>[2x]ATTYNAVVSKSSSDGKTFKTIADAIASAPAGST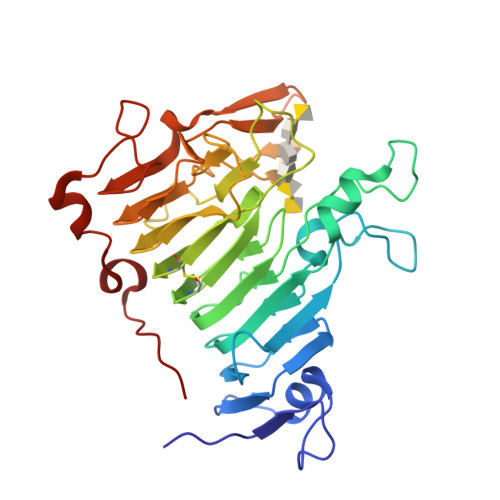PFVILIKNGVYNERLTITRNNLHLKGESRNGAVIAAATAAGTLKSDGSKWGTAGSSTITISAKDFSAQSLTIRNDFDFPANQAKSDSDSSKIKDTQAVALYVTKSGDRAYFKDVSLVGYQATLYVSGGRSFFSDCRISGTVDFIFGDGTALFNNCDLVSRYRADVKSGNVSGYLTAPSTNINQKYGLVITNSRVIRESDSVPAKSYGLGRPWHPTTTFSDGRYADPNAIGQTVFLNTSMDNHIYGWDKMSGKDKNGNTIWFNPEDSRFFEYKSYGAGATVSKDRRQLTDAQAAEYTQSKVLGDWTPTLP>MSSLSRELVFLILQFLDEEKFKETVHKLEQESGFFFNMKYFEEKVHAGEWDEVEKYLSGFTKVDDNRYSMKIFFEIRKQKYLEALDRHDRAKAVDILVKDLKVFSTFNEELYKEITQLLTLENFRENEQLSKYGDTKSARSIMLIELKKLIEANPLFREKLVFPTLKASRLRTLINQSLNWQHQLCKNPRPNPDIKTLFTDHTCTPPNG[2x];>[2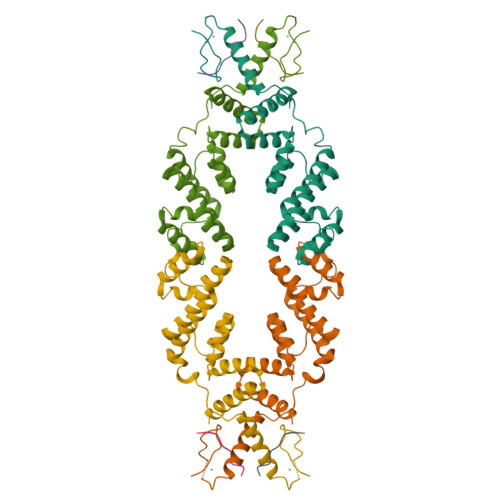x]DNLIYLDLNLQDWDD> PYVRLGYEGILNGAHDIDVAGLNGVEQLAGKFATIGANGVKLAGDNGTNAVGLFREDLGDMVNASEKASFYFRGGEYYVNISRTSL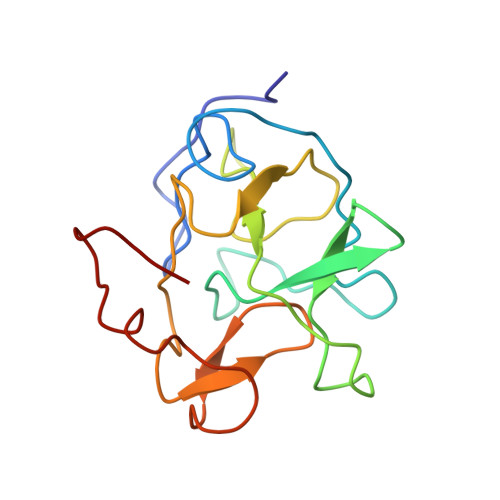TAAGIAAGDEITCDADGKMIKFTGTGKALGVVTHVGEYRAGNMYEKATQGVTDTDTFIGFIMYV N-(3-{[(2,6-dimethylphenyl)methyl]amino}-7-methoxyindeno[1,2-c]pyrazol-6-yl)methanesulfonamide | C21 H22 N4 O3 S | 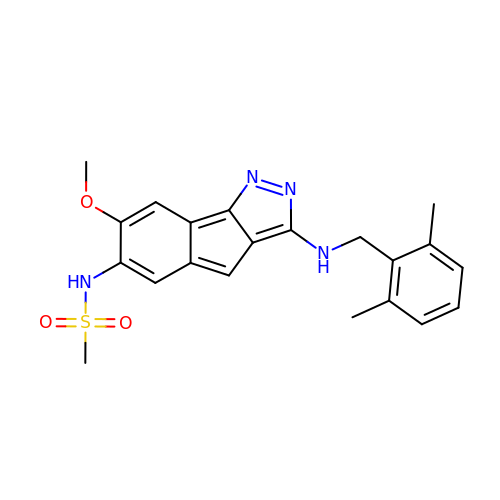YLMQFWXDIVNPGV-UHFFFAOYSA-N4-[2-(phenylsulfanyl)ethyl]morpholine | C12 H17 N O S | 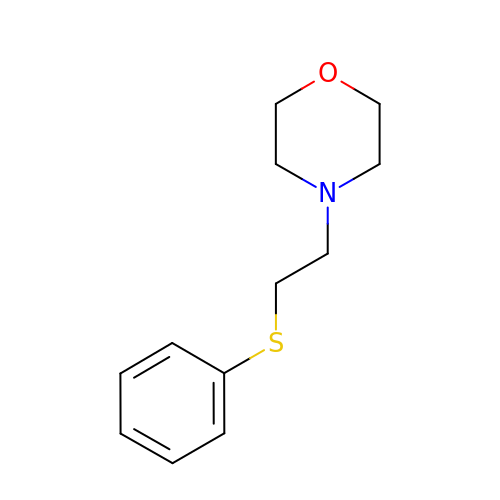QDTNFZGZGSMNCU-UHFFFAOYSA-N>MAEAAAAAAAAAAAGETSASSGSAAERDPDQDRAGRRLRVLSGHLLGRPQEALSTNECKARRAASAATAAPTATPAAPESGIIPKKRQELMKWNGWGYNDSKFFLNKKGQLELTGKRYPLSGVALPTFKDWIQNTFGINLDHKTTSKASLNPSDTPPSIVNEDFLHELKKTNISYSQEADDRVFRAHGHCLHEIFLLREGMFERIPDIVLWPTCHDDVVKIVNLACKYNLCIIPIGGGTSVSYGLMCPADETRTIISLDTSQMNRILWVDENNLTAHVEAGITGQELERQLKESGYCTGHEPDSLEFSTVGGWISTRASGMKKNIYGNIEDLVVHMKVVTPRGVIEKSCQGPRMSTGPDIHHFIMGSEGTLGVITEATIKIRPTPEYQKYGSVAFPNFEQGVACLREIAKQRCAPASIRLMDNQQFQFGHALKPQVSSIFTSFLDGLKKFYITKFKGFDPNQLSVATLLFEGDREKVLQHEKQVYDIAAKFGGLAAGEDNGQRGYLLTYVIAYMR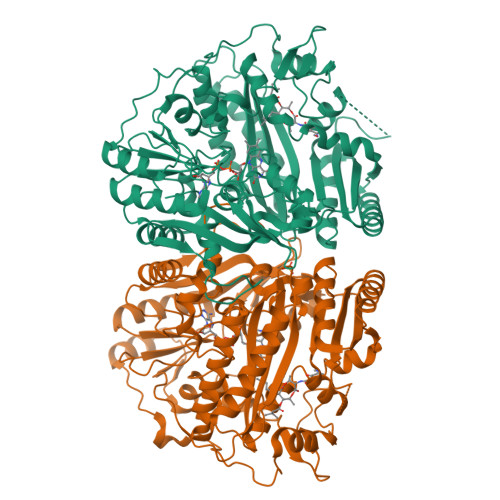DLGLEYYIIGESFETSAPWDRVVDLCRNVKERIRRECKEKGVQFPPLSTCRVTQTYDAGACIYFYFAFNYRGISDPLAVFEQTEAAAREEILANGGSLSHHHGVGKLRKQWLKESISDVGFGMLKSVKDYVDPTNIFGNRNLL[4x]In Gram-positive Firmicutes, it also has a role in natural transformation, while in Gram-negative bacteria, ComM is the canonical transformation-specific helicase. Comprehensive biochemical characterization of RadA from Escherichia coli, S. pneumoniae, B. subtilis and Thermus thermophilus and ComM from V. cholerae revealed that they are functional homologs during HR. Both RadA and ComM were found to be ring-shaped hexameric DNA motors powered by ATP hydrolysis to direct three-stranded DNA branch migration in vitro. Here, we present and compare the cryoEM (cryogenic electron microscopy) structures of RadA and ComM from S. pneumoniae and Legionella pneumophila, respectively, in interaction with DNA.

RadA from S. pneumoniae was purified from E. coli mainly as a hexamer and shown to exhibit ATPase activity in the presence of DNA, with lower activity on dsDNA than on ssDNA. To gain a better understanding of the interaction between RadA and DNA, purified RadA was incubated in the presence of the poorly hydrolyzable ATP analog ATPγS with a gapped DNA substrate consisting of 30 base pairs (bps) of dsDNA followed by 60 nucleotides (nts) of ssDNA and 30 bp of dsDNA (Combination CD in Appendix Table S1). Density maps of hexameric RadA bound to DNA were obtained using cryoEM, yielding a resolution of 3.15 Å. Strikingly, the ATPase domains adopt a helical configuration in the dsDNA-bound RadA structure. In the CryoEM structure of DNA-bound RadA, the Lon domain has planar and hexameric ring-shaped C6 symmetry as in the DNA-free crystal structure of RadA. The flexible linker connecting the Lon and ATPase domains allows for this symmetry mismatch. Here, we reveal a cryoEM structure of the RadA hexamer bound to dsDNA with five ATPase active sites occupied by ATP-γ-S and the last unoccupied. Upon interaction with dsDNA, the ATPase domains adopt a helical organization. This places the KNRFG motif, which includes both the arginine finger and the catalytic piston, in close proximity to the bound ATP molecule of the neighboring subunit. The primary contact with DNA is established by K216, which binds to the phosphate of the DNA backbone and coordinates the 5’ to 3’ DNA strand (ZF to Lon domain polarity) in a manner similar to that of DnaB loops. A second region corresponding to the N-terminus of the helix 188–204, named RH1 (RadA helix 1), coordinates the complementary DNA strand. In the CryoEM structure, R301 is involved in a salt bridge with either E76 or E239 in the most retracted or stretched subunits, respectively.

>[6x]MASWSHPQFEKSGGGGGLVPRGSKKKATFVCQNCGYNSPKYLGRCPNCGSWSSFVEEVEVAEVKNARVSLTGEKTKPMKLAEVTSINVNRTKTEMEEFNRVLGGGVVPGSLVLIGGDPGIGKSTLLLQVSTQLSQVGTVLYVSGEESAQQIKLRAERLGDIDSEFYLYAETNMQSVRAEVERIQPDFLIIDSIQTIMSPEISGVQGSVSQVREVTAELMQLAKTNNIAIFIVGHVTKEGTLAGPRMLEHMVDTVLYFEGERHHTFRILRAVKNRFGSTNEIGIFEMQSGGLVEVLNPSQVFLEERLDGATGSSIVVTMEGTRPILAEVQALVTPTMFGNAKRTTTGLDFNRASLIMAVLEKRAGLLLQNQDAYLKSAGGVKLDEPAIDLAVAVAIASSYKDKPTNPQECFVGELGLTGEIRRVNRIEQRINEAAKLGFTKIYVPKNSLTGITLPKEIQVIGVTTIQEVLKKVF> MASIKKVYRGMKNGAETINDDLEAINSELTSGGNVVHKTGDETIAGKKTFTGNVEVNGSLTL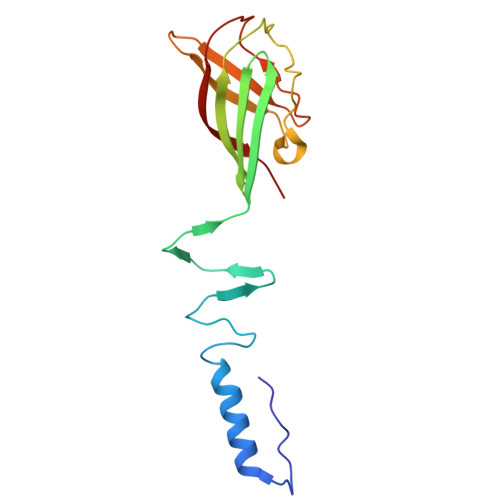PTKSWSGELGGGIILSLRKKGTTVEYSIGGEISSSILANSNLVNRSVPNEFCPRNRCSLVGHMVGGWNAFHIDIPSSGVCQWFGPTASSGTPRGTGTYPIDH> APTGDPACRAAVATAQKIAPLAHGEVAALTMASAPLKLPDLAFEDADGKPKK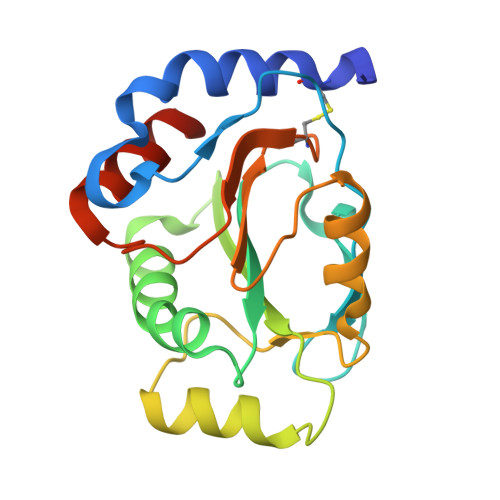LSDFRGKTLLVNLWATWCVPSRKEMPALDELQGKLSGPNFEVVAINIDTRDPEKPKTFLKEANLTRLGYFNDQKAKVFQDLKAIGRALGMPTSVLVDPQGCEIATIAGPAEWASEDALKLIRAATGKAAAAL> MGHHHHHHHHHHSSGHIEGRH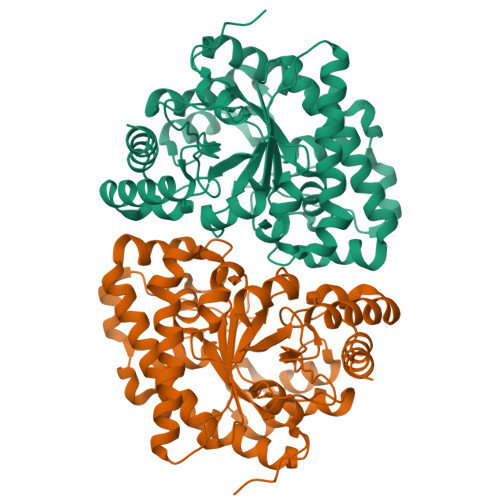MEANGLGPQGFPELKNDTFLRAAWGEETDYTPVWCMRQAGRYLPEFRETRAAQDFFSTCRSPEACCELTLQPLRRFPLDAAIIFSDILVVPQALGMEVTMVPGKGPSFPEPLREEQDLERLRDPEVVASELGYVFQAITLTRQRLAGRVPLIGFAGAPWTLMTYMVEGGGSSTMAQAKRWLYQRPQASHQLLRILTDALVPYLVGQVVAGAQALQLFESHAGHLGPQLFNKFALPYIRDVAKQVKARLREAGLAPVPMITFAKDGHFALEELAQAGYEVVGLDWTVAPKKARECVGKTVTLQGNLDPCALYASEEEIGQLVKQMLDDFGPHRYIANLGHGLYPDMDPEHVGAFVDAVHKHSRLLRQN>[2x]DPSKDSKAQVSAAEAGITGTWYNQLGSTFIVTAGADGALTGTYESAVGNAESRYVLTGRYDSAPATDGSGTALGWTVAWKNNYRNAHSATTW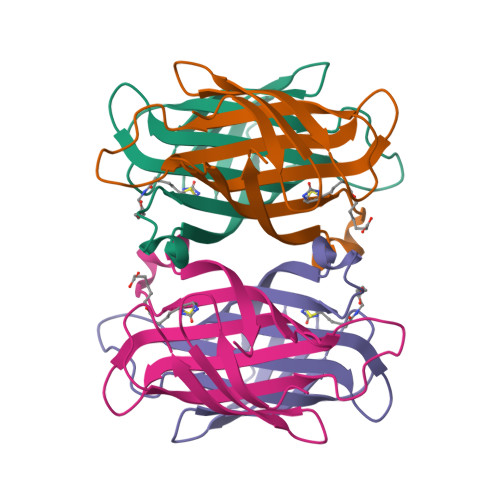SGQYVGGAEARINTQWLLTSGTTEANAWKSTLVGHDTFTKVKP> MFENITAAPADPILGLADLFRADERPGKINLGIGVYKDETGKTPVLTSVKKAEQYLLENETTKNYLGIDGIPEFGRCTQELLFGKGSALINDKRARTAQTPGGTGALRVAADFLAKNTSVKRVWVSNPSWPNHKSVFNSAGLEVREYAYYDAENHTLDFDALINSLNEAQAGDVVLF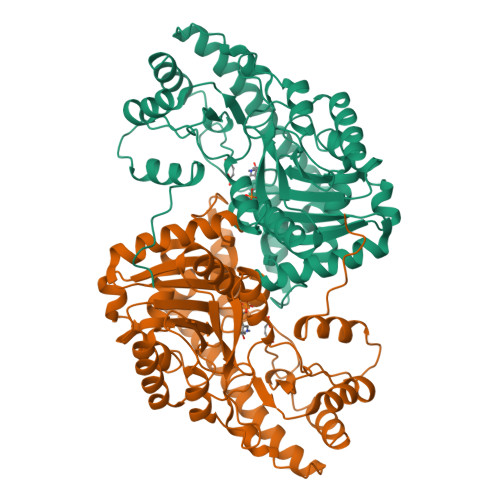HGYCHNPTGIDPTLEQWQTLAQLSVEKGWLPLFDFAYQGFARGLEEDAEGLRAFAAMHKELIVASSYSKNFGLYNERVGACTLVAADSETVDRAFSQMKAAIRANYSNPPAHGASVVATILSNDALRAIWEQELTDMRQRIQRMRQLFVNTLQEKGANRDFSFIIKQNGMFSFSGLTKEQVLRLREEFGVYAVASGRVNVAGMTPDNMAPLCEAIVAVL>[2x]GMRGLIVDYAGVLDGTDEDQRRWRNLLAAAKKNGVGTVILSNDPGGLGAAPIRE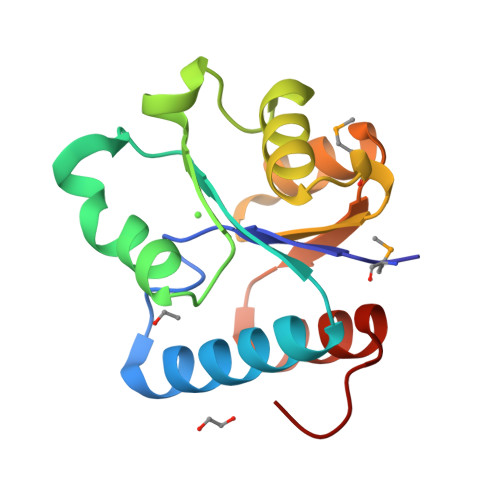LETNGVVDKVLLSGELGVEKPEEAAFQAAADAIDLPMRDCVLVDDSILNVRGAVEAGLVGVYYQQFDRAVVEIVGLFGLEGEF>[4x]MEMGRRIHLELRNRTPSDVKELVLDNSRSNEGKLEGLTDEFEELEFLSTINVGLTSIANLPKLNKLKKLELSDN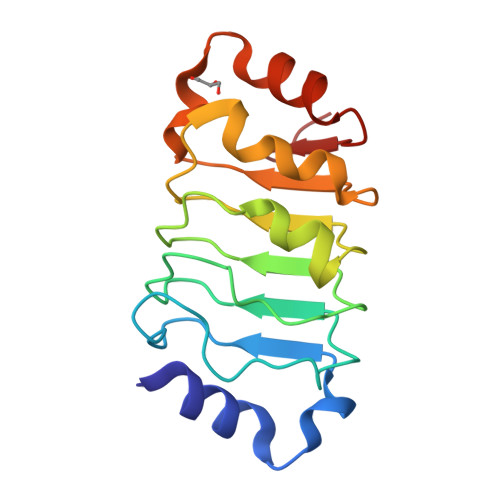RVSGGLEVLAEKCPNLTHLNLSGNKIKDLSTIEPLKKLENLKSLDLFNCEVTNLNDYRENVFKLLPQLTYLDGYD> MNSENTIVYVRVAGRARNGFVDPLKFYWDLERDRSLWSSV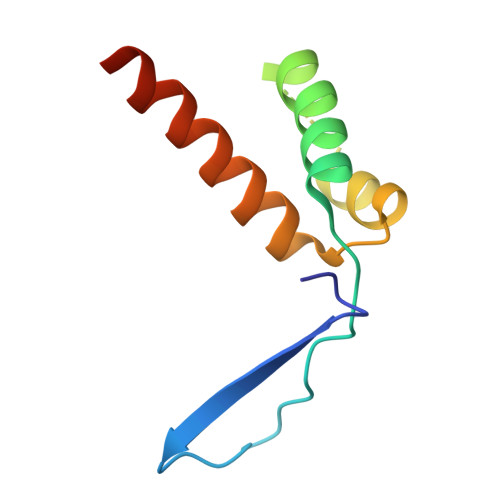SKLDNTKKTIDWKRLSREFKAPEHFIRKRSYALFAKHLKLLERQIEA>[2x]SNADEVQVAVAANFTAPIQAIAKEFEKDTGHRLVAAYGATGQFYTQIKNGAPFQVFLSADDSTPAKLEQEGEVVPGSRFTYAIGTLALWSPKAGYVDAEGEVLKSGSFRHLSIANPKTAPYGLAATQAMDKLGLAATLGPKLVEGQNISQAYQFVSSGNAELGFVALSQIYKDGKVATGSAWIVPTELHDPIRQDAVILNKGKDNAAAKALVDYLKGAKAAALIKSYGYEL

Acquisition of the trace-element molybdenum via the high-affinity ATP-binding cassette permease ModABC is essential for Pseudomonas aeruginosa respiration in anaerobic and microaerophilic environments. Molybdenum, which predominantly occurs as the oxyanion molybdate (MoO42−; henceforth MoO), is imported via the high-affinity ATP-binding cassette (ABC) permease, ModABC in P. aeruginosa. Pseudomonas aeruginosa PAO1 ModA has a non-contiguous dual-hinged bilobal structure with a single metal-binding site positioned between the two domains.

Metal binding results in a 22° relative rotation of the two lobes with the oxyanions coordinated by four residues, that contribute six hydrogen bonds, distinct from ModA orthologues that feature an additional oxyanion-binding residue. Analysis of 485 Pseudomonas ModA sequences revealed conservation of the metal-binding residues and β-sheet structural elements, highlighting their contribution to protein structure and function.>MSKTTSNAGLNLIKGFEGKRLNAYDDGVGVWTIGFGTIKYPNGVRVKKGDTCTEQQAETYLKNDLTKFEVAINKLVKVSLTQNQFDALASFTYNLGETNLANSTLLKKLNKGDYQGAADQFLVWNKAGGKVMKGLVRRREAERALFLK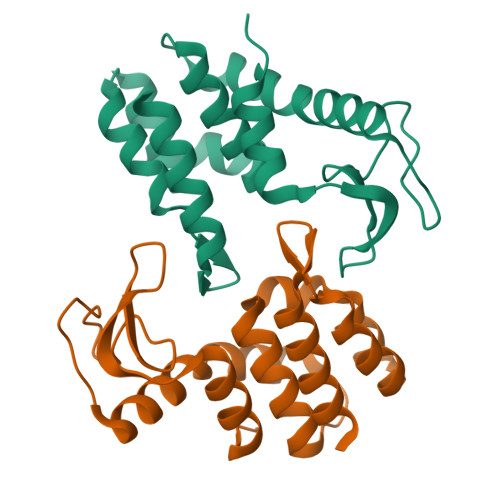K[2x]>MSKIVKIIGREIIDSRGNPTVEAEVHLEGGFVGMAAAPSGASTGSREALELRDGDKSRFLGKGVTKAVAAVNGPIAQALIGKDAKDQAGIDKIMIDLDGTENKSKFGANAILAVSLANAKAAAAAKGMPLYEHIAELNGTPGKYSMPVPMMNIINGGEHADNNVDIQEFMIQPVGAKTVKEAIRMGSEVFHHLAKVLKAKGMNTAVGDEGGYAPNLGSNAEALAVIAEAVKAAGYELGKDITLAMDCAASEFYKDGKYVLAGEGNKAFTSEEFTHFLEELTKQYPIVSIEDG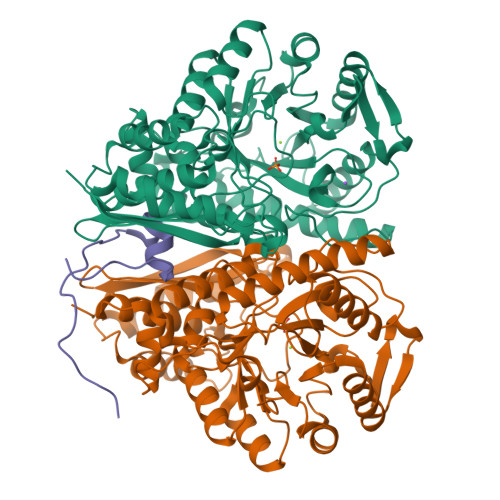LDESDWDGFAYQTKVLGDKIQLVGDDLFVTNTKILKEGIEKGIANSILIKFNQIGSLTETLAAIKMAKDAGYTAVISHRSGETEDATIADLAVGTAAGQIKTGSMSRSDRVAKYNQLIRIEEALGEKAPYNGRKEIKGQA[4x];> RRYRDERYPTQSPMPLTVACASPELASGKVWIRYPI;> RDERYPTQSPMPLTVACASPELASGKVWIRYPIVR(1H-pyrazol-4-yl)(pyrrolidin-1-yl)methanone | C8 H11 N3 O | 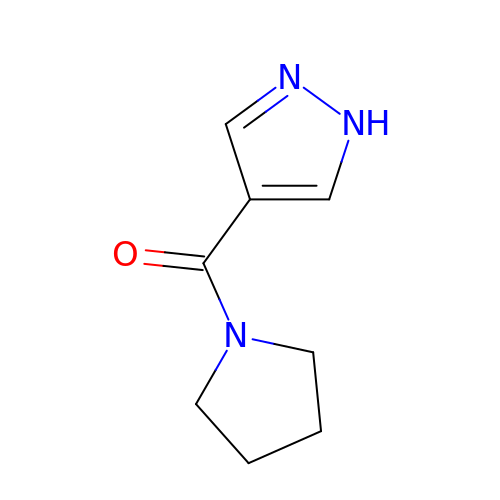ZCTYYKNBCKBIMR-UHFFFAOYSA-N> MTKKGDTYNEAWVKDTNGFDILMGQFAHNIENIWGFKEVVIAGPKDYVKYT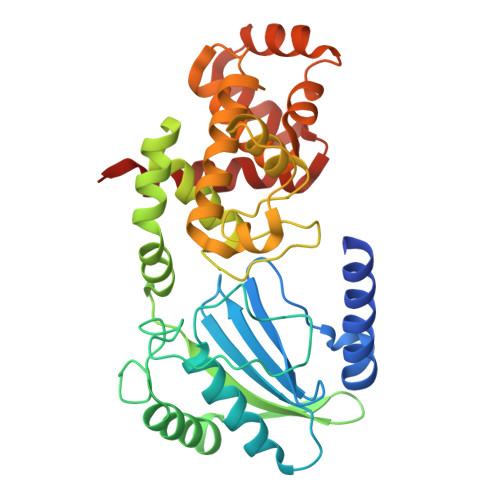DQYQTRSHINFDDGTITIETIAGTEPAAHLRRAIIKTLLMGDDPSSVDLYSDVDDITISKEPFLYGQVVDNTGQPIRWEGRASNFADYLLKNRLKSRSNGLRIIYSVTINMVPNHLDKRAHKYLGMVRQASRKYGVDESLILAIMQTQSSFNPYAVSRSDALGLMQVVQHTAGKDVFRSQGKSGTPSRSFLFDPASNIDTGTAYLAMLNNVYLGGIDNPTSRRYAVITAYNGGAGSVLRVFSNDKIQAANIINTMTPGDVYQTLTTRHPSAESRRYLYKVNTAQKSYRRR>MNNKSLLYPVVSTSRRVVSLDGMWRFSFDAKSEGVEANWANGLPESISMPVPASFCDFFTDKESREYCGDFWYETDFFVPGEWSGKDIAIRFGSATHHARIFVNGVEVAQHEGGFLPFDAVVTDIVRYNQFNKLSVLLNNELNEHMLPAGNTAVLSNGKKVAAPYFDFYNYAGIHRPVKLMALPTERILDYSVKHRLTAEGAEVDYTVTTNGDHEVTVELYDGTTKVAEATGKEGTLVVKDAKLWNVHAAYLYNIVIRIHDGSAVVDEYTEKVGIRTFEIKDGHFLLNGKPVYLRGFGKHEDADIRGRGLDLATVKRDYELMKWIGANCFRTSHYPYAEELYQMADEEGFLIIDEVPAVGFMESTMNFLAANQGNGKKVGWFEKETTPQLLANHKDALTDMIGRDKNHASVIAWSILNEPQCTSEGTEAYFKTLFDLAHELDPQKRPRTYAVVMMSLPNNSKGQQFADFISLNRYYGWYVMGGMGIVDAEAAFRKEMNGWAQVLNGRPMIFTEYGADTMPTEHKLPSVM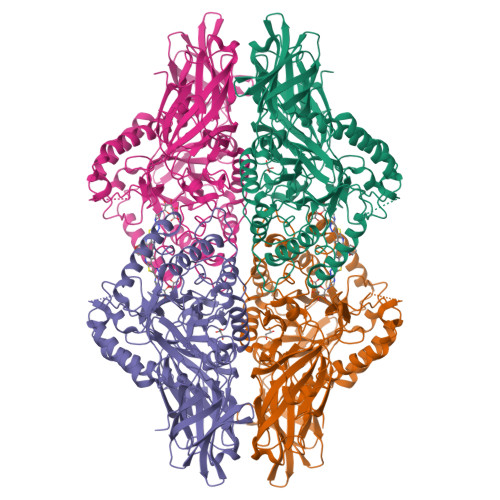WSQEYQNEYLDMNHNVFDSYNFVQGELVWNFADFQTTEGILRVNGNKKGIFTRQRQPKDAAFLFRARWTSLPLDYKGNQ[4x]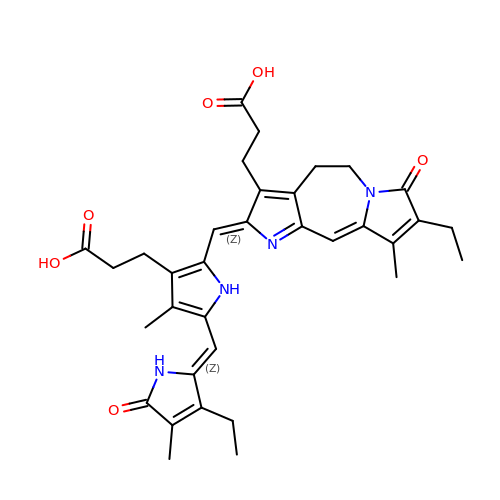3-[2-[(~{Z})-[12-ethyl-6-(3-hydroxy-3-oxopropyl)-13-methyl-11-oxidanylidene-4,10-diazatricyclo[8.3.0.0^{3,7}]trideca-1,3,6,12-tetraen-5-ylidene]methyl]-5-[(~{Z})-(3-ethyl-4-methyl-5-oxidanylidene-pyrrol-2-ylidene)methyl]-4-methyl-1~{H}-pyrrol-3-yl]propanoic acid | C34 H38 N4 O6 | ZPENGPJFMYEJSJ-DPTABBBISA-N>MSSRKVSRAHYDEDELASAANMSLVAEGHFRGMKELLSTMDLDTDANTIPELKERAHMLCARFLGGAWKTVPLEHLRISRIKGGMSNMLFLCRLSEVYPPIRNEPNKVLLRVYFNPETESHLVAESVIFTLLSERHLGPKLYGIFSGGRLEEYIPSRPLSCHEISLAHMSTKIAKRVAKVHQLEVPIWKEPDYLCEALQRWLKQLTGTVDAEHRFDLPEECGVSSVNCLDLARELEFLRAHISLSKSPVTFCHNDLQEGNILLPKASSGNIRMPSLSDETQALGNSLSAFNPADP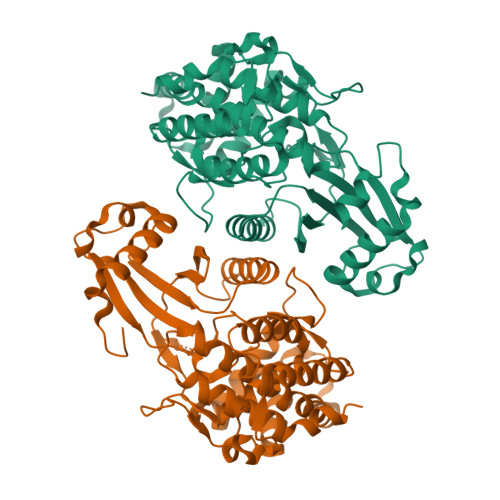RLVLIDFEYASYNYRAFDFANHFIEWTIDYDIDEAPFYKIQTENFPENDQMLEFFLNYLREQGNTRENELYKKSEDLVQETLPFVPVSHFFWGVWGLLQVELSPVGFGFADYGRDRLSLYFKHKQLLKNLASHQ[2x]1,2,3,4-TETRAHYDRO-ISOQUINOLINE-7-SULFONIC ACID AMIDE | C9 H12 N2 O2 S | 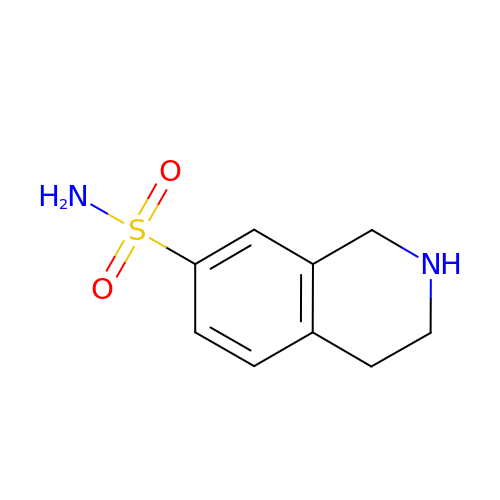UGLLZXSYRBMNOS-UHFFFAOYSA-N>[4x]SDKIIHLTDDSFDTDVLKADGAILVDFWAEWCG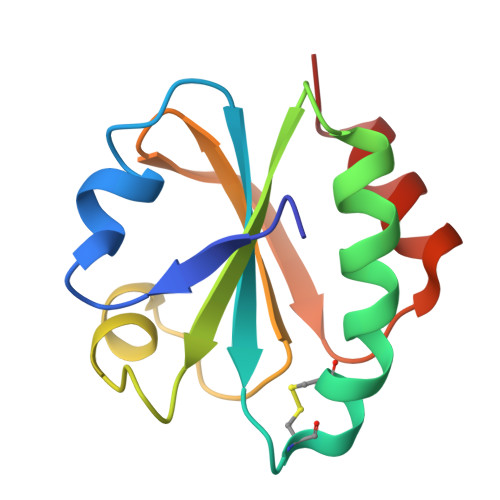PCKMIAPILDEIADEYQGKLTVAKLNIDQNPGTAPKYGIRGIPTLLLFKNGEVAATKVGALSKGQLKCFLDANLA> YKDGDQCETSPCQNQGKCKDGLGEYTCTCLEG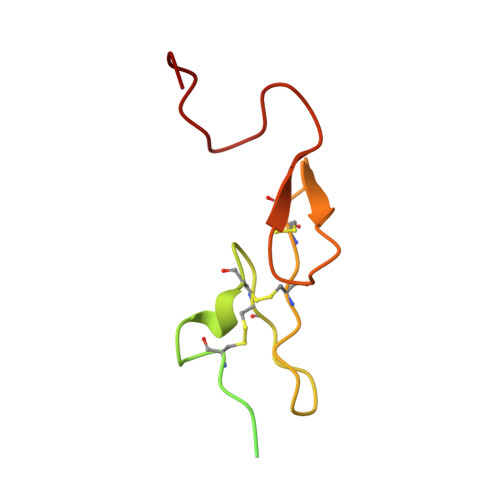FEGKNCELFTRKLCSLDNGDCDQFCHEEQASVVCSCARGYTLADNGKACIPTGPYPCGKQTLER> MVSSVLEVSHVFCCPNRVRGALSWNTGPGGLLAFGTSCSVVLYDPQKKVVITNLNGHTARVNCLQWIRTEDGSPSNELVSGGSDNRVIHWELENNQVLKSVRLQGHEGPVCAVHAIYQSGPSEGEQHALIASAASDSTVRIWSKKGSEVKYLQTLSFRDGFVLSVCLAILPGTNVPVLACGDDDCRIHLYIQQDDQFQKALSLCGHEDWIRGVEWATFGRDLFLASCSQDCLIRIWRLYMKPASFETKDGSLRLKENTFTIKDGGVRTTVAVTLETVLAGHENWVNAVHWQPSFYKDGVLQQPVRLLSASMDKTMILWAPDEESGVWLEQVRVGEVGGNTLGFYDCQFGENGTMIIAHAFHGALHLWKQSTVNPRQWAPEIVISGHFDGVQDLMWDPEGEFIITTSTDQTTRLFAPWKKKDQKDRSQVTWHEIARPQIHGYNIKCLAMIDRFQFVSGADEKVLRVFSAPRNFVENFSVISRQSLSHMLCDDQDLPEGATVPALGLSNKALFQGDIASQPFEEDELISPAFGSPQVTFQPAVLNEPPTEDHLLQNTLWPEIQKLYGHGYEIVCVACNNSKTLLASACKASQKEHAAIILWSTASWKQVQSLAFHTLTVTQMTFSPDDKFLLAVSRDRTWSLWKRQDATSSEFDPFFSLFAFTNKITSVHSRIIWSCDWSPDNKYFFTGSRDKKVVVWGECKSSHNPMEHPIRPCSSILDVGSSVTAVSVCPVLNPAQRYIVAIGLESGKICIYSWNKTNQEINDWTSCVETNPSQSHSLGIRRLCWKSCSDDDDDDDDDDTEQSEEG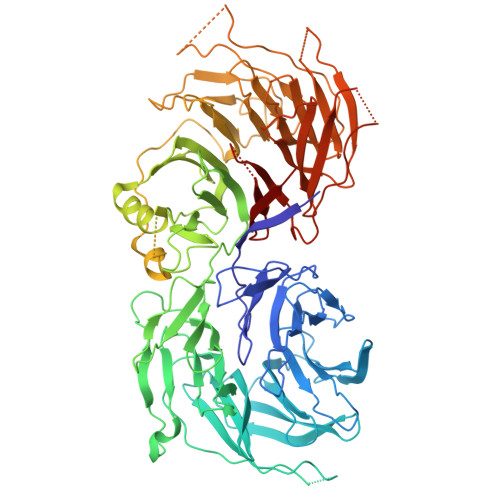PEWLHFASCGEDHTVKIYRVNRRAL> MTRDEMISVEPEAAELQDQHRRDFLKRSGAAVLSLSLSSLATGVVPGFLKDAQAGTKAPGYASWEDIYRKEWKWDKVNWGSHLNICWPQGSCKFYVYVRNGIVWREEQAAQTPACNVDYVDYNPLGCQKGSAFNNNLYGDERVKYPLKRVGKRGEGKWKRVSWDEAAGDIADSIIDSFEAQGSDGFILDAPHVHAGSIAWGAGFRMTYLMDGVSPDINVDIGDTYMGAFHTFGKMHMGYSADNLLDAELIFMTCSNWSYTYPSSYHFLSEARYKGAEVVVIAPDFNPTTPAADLHVPVRVGSDAAFWLGLSQVMIDEKLFDRQFVCEQTDLPLLVRMDTGKFLSAEDVDGGEAKQFYFFDEKAGSVRKASRGTLKLDFMPALEGTFSARLKNGKTIQVRTVFEGLREHLKDYTPEKASAKCGVPVSLIRELGRKVAKKRTCSYIGFSSAKSYHGDLMERSLFLAMALSGNWGKPGTGAFAWAYSDDNMVYLGVMSKPTAQGGMDELHQMAEGFNKRTLEADPTSTDEMGNIEFMKVVTSAVGLVPPAMWLYYHVGYDQLWNNKAWTDPALKKSFGAYLDEAKEKGWWTNDHIRPAPDKTPQVYMLLSQNPMRRKRSGAKMFPDVLFPKLKMIFALETRMSSSAMYADIVLPCAWYYEKHEMTTPCSGNPFFTFVDRSVAPPGECREEWDAIALILKKVGER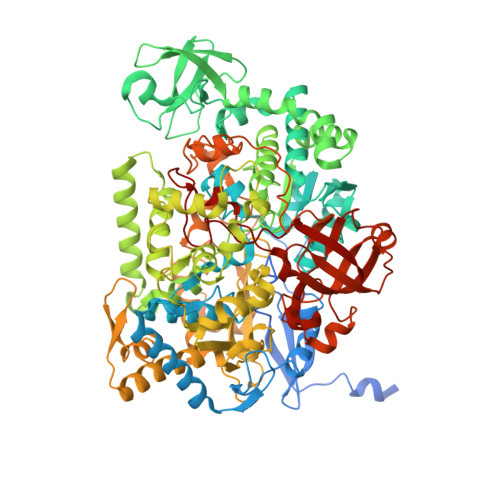AAARGLTEFNDHNGRKRRYDELYKKFTMDGHLLTNEDCLKEMVDINRAVGVFAKDYTYEKFKKEGQTRFLSMGTGVSRYAHANEVDVTKPIYPMRWHFDDKKVFPTHTRRAQFYLDHDWYLEAGESLPTHKDTPMVGGDHPFKITGGHPRVSIHSTHLTNSHLSRLHRGQPVVHMNSKDAAELGIKDGDMAKLFNDFADCEIMVRTAPNVQPKQCIVYFWDAHQYKGWKPYDILLIGMPKPLHLAGGYEQFRYYFMNGSPAPVTDRGVRVSIKKA> MASIKKVYRGMKNGAETINDDLEAINSELTSGGNVVHKTGDETIAGKKTFTGNVEVNGSLTLPTKSWSGELGGGIILSLRKKGTT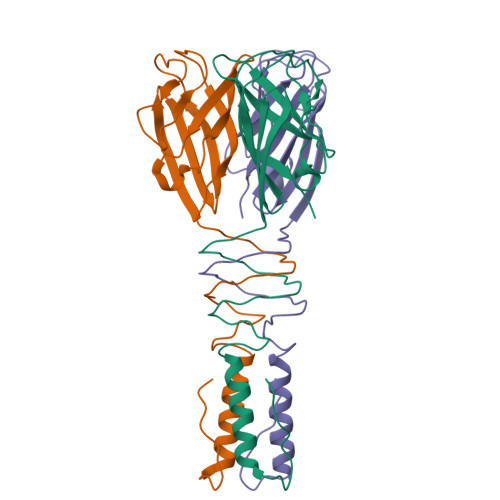VEYSIGGEISSSILANSNLVNRSVPNEFCPRNRCSLVGHMVGGWNAFHIDIPSSGVCQWFGPTASSGTPRGTGTYPIDHHHHHH>MASGV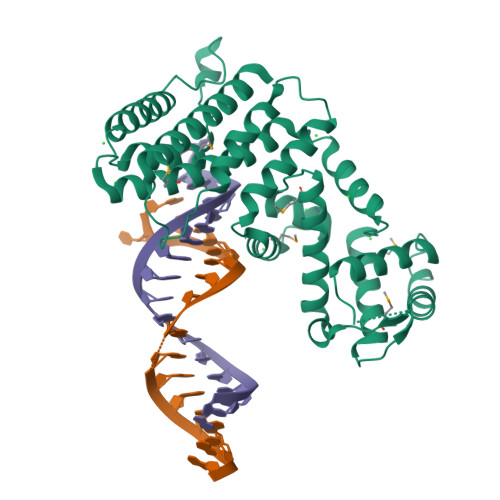EDTKHYEEAKKCVEELALYLKPLSSARGVGLNSTTQSVLSRPMQRKLVTLVHCQLVEEEGRIRAMRAARSLGERTVTELILQHQNPQQLSSNLWAAVRARGCQFLGPAMQEEALKLVLLALEDGSALSRKVLVLFVVQRLEPRFPQASKTSIGHVVQLLYRASCFKVTKRDEDSSLMQLKEEFRTYEALRREHDSQIVQIAMEAGLRIAPDQWSSLLYGDQSHKSHMQSIIDKLQTPASFAQSVQELTIALQRTGDPANLNRLRPHLELLANIDPSPDAPPPTWEQLENGLVAVRTVVHGLVDYIQNHSKKGADQQQLEHHHHHH[2x]> APLVHHHHHHALDENLYFQGALADVSRPPHARKTGGSSPETKYDQPPKCDISGKEAISALSRAKSKHCRQEIGETYCRHKLGLLMPEKVTRFCPLEGKANKNVQWDEDSVEYMPANPVRIAFVLVVHGRASRQLQRMFKAIYHKDHFYYIHVDKRSNYLHRQVLQVSRQYSNVRVTPWRMATIWGGASLLSTYLQSMRDLLEMTDWPWDFFINLSAADYPIRTNDQLVAFLSRYRDMNFLKSHGRDNARFIRKQGLDRLFLECDAHMWRLGDRRIPEGIAVDGGSDWFLLNRRFVEYVTFSTDDLVTKMKQFYSYTLLPAESFFHTVLENSPHCDTMVDNNLRITNW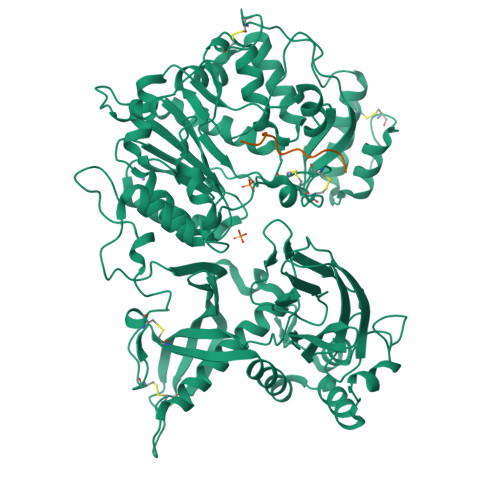NRKLGCKCQYKHIVDWCGCSPNDFKPQDFHRFQQTARPTFFARKFEAVVNQEIIGQLDYYLYGNYPAGTPGLRSYWENVYDEPDGIHSLSDVTLTLYHSFARLGLRRAETSLHTDGENSCRYYPMGHPASVHLYFLADRFQGFLIKHHATNLAVSKLETLETWVMPKKVFKIASPPSDFGRLQFSEVGTDWDAKERLFRNFGGLLGPMDEPVGMQKWGKGPNVTVTVIWVDPVNVIAATYDILIESTAEFTHYKPPLNLPLRPGVWTVKILHHWVPVAETKFLVAPLTFSNRQPIKPEEALKLHNGPLRNAYMEQSFQSLNPVLSLPINPAQVEQARRNAASTGTALEGWLDSLVGGMWTAMDICATGPTACPVMQTCSQTAWSSFSPDPKSELGAVKPDGRLR;> QEPEGSGGGQG> MASWSHPQFEKGALEDPRSLYDLPPYGDATLLYFSDLHGQAFPHYFMEPPNLIAPKPLMGRPGYLTGEAILRYYGVERGTPLAYLLSYVDFVELARTFGPIGGMGALTALIRDQKARVEAEGGKALVLDGGDTWTNSGLSLLTRGEAVVRWQNLVGVDHMVSHCEWTLGRERVEELLGLFRGEFLSYNIVDDLFGDPLFPAYRIHRVGPYALAVVGASYPYVKVSHPESFTEGLSFALDERRLQEAVDKARAEGANAVVLLSHNGMQLDAALAERIRGIDLILSGHTHDLTPRPWRVGKTWIVAGSAAGKALMRVDLKLWKGGIANLRVRVLPVLAEHLPKAEDVEAFLKAQLAPHQDHLFTPLAVSETLLYKRDTLYSTWDQLVGEAVKAIYPEVEVVFSPAVRWGTTILPGQAITWDHLYAYTGFTYPELYLFYLRGAQIKAVLEDIASNVFTSDPFYQQGGDVSRVFGLRYV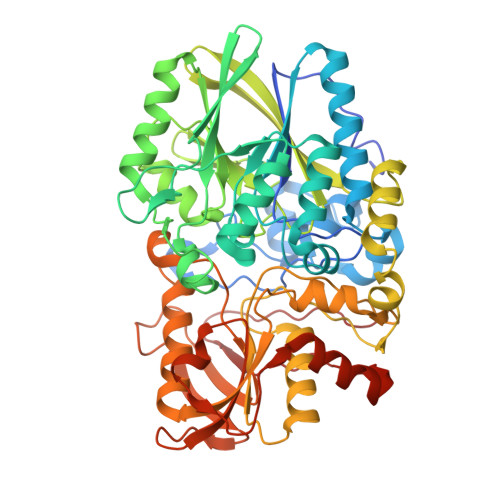LDPDAPTGERVREVEVGGRPLDPNRRYLAAAYGGRLQRVGEAKPGYEPRPIYEVLAEYLRSVGRVRVRPEPNVKVIGRNYRLPEVTG>MGSSHHHHHHSSGENLYFQGHMHEEENVVRSNIDISKISGEWYSILLASDVKEKIEENGSMRVFVEHIKALDNSSLSFVFHTKENGKCTEIFLVADKTKDGVYTVVYDGYNVFSIVETVYDEYILLHLLNFDKTRPFQLVEF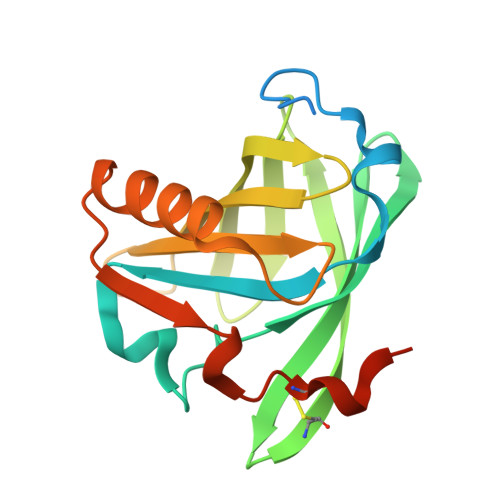YAREPDVSQKLKEKFVKYCQEHGIVNILDLTEVDRCLQARGSEVAQDSSVE[4x]> AVSLDRTRAVFDGSEKSMTLDISNDNKQLPYLAQAWIENENQEKIITGPVIATPPVQRLEPGAKSMVRLSTTPDISKLPQDRESLFYFNLREIPPRSEKANVLQIALQTKIKLFYRPAAIKTRPNEVWQDQLILNKVSGGYRIENPT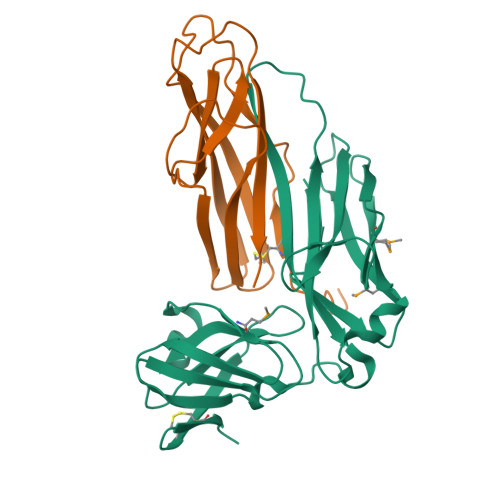PYYVTVIGLGGSEKQAEEGEFETVMLSPRSEQTVKSANYNTPYLSYINDYGGRPVLSFICNGSRCSVKKEK;> HHHHHHGGCRPSAQSLEIKHGDLSINSANNHYAAQTLSVSCDVPANIRFMLLRNTTPTYSHGKKFSVGLGHGWDSIVSVNGVDTGETTMRWYKAGTQNLTIGSRLYGESSKIQPGVLSGSATLLMILP> GMWQFPLFETILIEQGQAKNISYHQQRYEKSLLKFYPKMKLQPFDLAKIIAKHTALFTHREGLIRCRID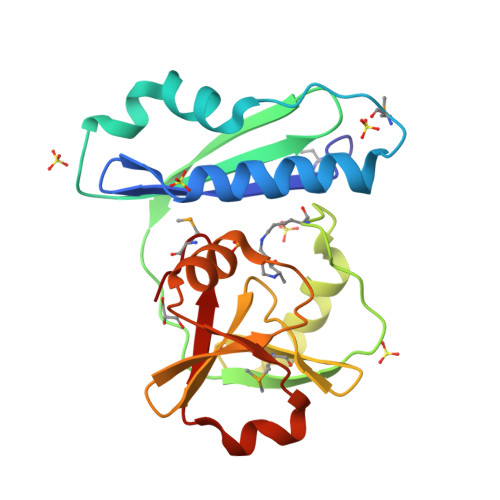YNHHDYVLQCFPYQQKVYRTFKPVFCDHIDYSLKFSDRTLLNNLLKQKEECDEIMIIRQGKVTDCSIGNLIFRQNNQWITPDKPLLEGTQRAKLLEQKKIIAREIFFEDLAQYEEIRLINAMNGL> MSFVDHPPDWLEEVGEGLREFLGLEAGPPKPKPNQQHQDQARGLVLPGYNYLGPGNGLDRGEPVNRADEVAREHDISYNEQLEAGDNPYLKYNHADAEFQEKLADDTSFGGNLGKAVFQAKKRVLEPFGLVEEGAKTAPTGKRIDDHFPKRKKARTEEDSKPSTSSDAEAGPSGSQQLQIPAQPASSLGADTMSAGGGGPLGDNNQGADGVGNASGDWHCDSTWMGDRVVTKSTRTWVLPSYNNHQYREIKSGSVDGSNANAYFGYSTPWGYFDFNRFHSHWSPRDWQRLINNYWGFRPRSLRVKIFNIQVKEVTVQDSTTTIANNLTSTVQVFTDDDYQLPYVVGNGTEGCLPAFPPQVFTLPQYGYATLNRDNGDNPTERSSFFCLEYFPSKMLRTGNNFEFTYSFEEVPFHCSFAPSQNLFKLANPLVDQYLYRFVSTSATGAIQFQKNLAGRYANTYKNWFPGPMGRTQGWNTSSGSSTNRVSVNNFSVSNRMNLEGASYQVNPQPNGMTNTLQGSNRYALENTMIFNAQNATPGTTSVYPEDNLLLTSESETQPVNRVAYNTGGQMATNAQNATTAPTVGTYNLQEVLPGSVWMERDVYLQGPIWAKIPETGAHFHPSPAMGGFGLKHPPPMMLIKNTPVPGNITSFSDVPVSSFITQYSTGQVTVEMEWELKKENSKRWNPEIQYTNNYNDPQFVDFAPDGSGEYRTTRAIGTRYLTRPL;> MASVSAGESVQITLPKNEVQLNAYVLQEPPKGETYTYDWQLITHPRDYSGEMEGKHSQILKLSKLTPGLYEFKVIVEGQNAHGEGYVNVTVKPEPRKNRPPIAIVSPQFQEISLPTTSTVIDGSQSTDDDKIVQYHWEELKGPLREEKISEDTAILKLSKLVPGNYTFSLTVVDSDGATNSTTANLTVNKAVDYPPVANAGPNQVITLPQNSITLFGNQSTDDHGITSYEWSLSPSSKGKVVEMQGVRTPTLQL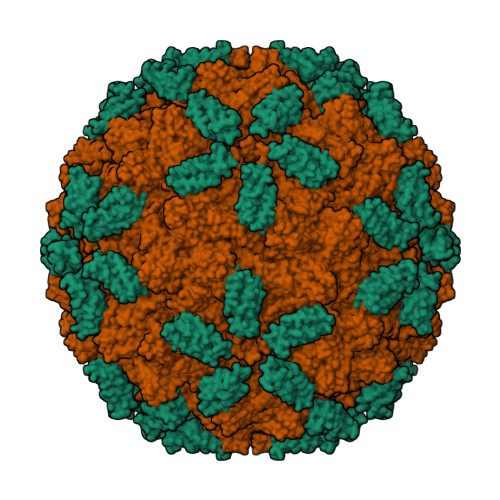SAMQEGDYTYQLTVTDTIGQQATAQVTVIVQPENNK>[4x]GSLVSYTP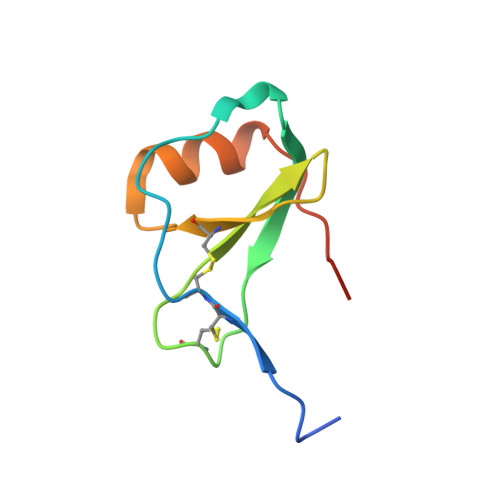NSCCYGFQQHPPPVQILKEWYPTSPACPKPGVILLTKRGRQICADPSKNWVRQLMQRLPAIAHHHHHH>[2x]GSDKIHHHHHHMQTFLKGKRVGYWLSEKKIKKLNFQAFAELCRKRGMEVVQLNLSRPIEEQGPLDVIIHKLTDVILEADQNDSQSLELVHRFQEYIDAHPETIVLDPLPAIRTLLDRSKSYELIRKIEAYMEDDRICSPPFMELTSLCGDDTMRLLEKNGLTFPFICKTRVAHGTNSHEMAIVFNQEGLNA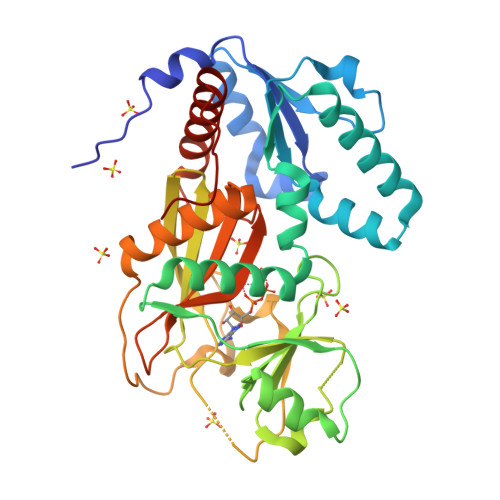IQPPCVVQNFINHNAVLYKVFVVGESYTVVQRPSLKNFSAGTSDRESIFFNSHNVSKPESSSVLTELDKIEGVFERPSDEVIRELSRALRQALGVSLFGIDIIINNQTGQHAVIDINAFPGYEGVSEFFTDLLNHIATVLQGQSTAMAATGDVAL> ADCTFTQLEIVPQFGSPNMFGGEDEHVRVMFSNEDPNDDNPDAFPEPPVYLADRDSGNDCRIEDGGIWSRGGVFLSQDGRRVLMHEFSGSSAELVSYDSATCKVVHREDISGQRWAVDKDGLRLGQKCSGESVDSCAKIV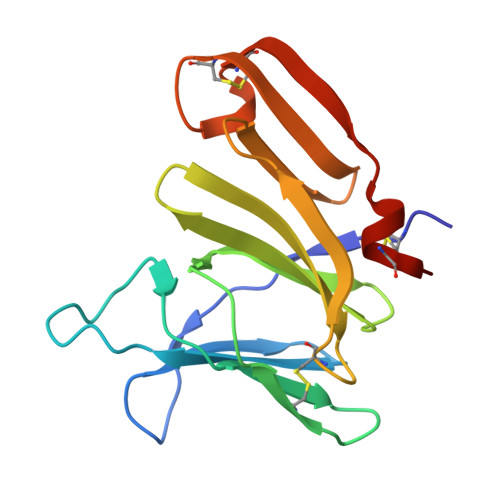KRSLAPFCQTAKK> SMGKAPVDPECTAKVGKAHVYCEGNDVYDVMLNQTNLQFNNNKYYLIQLLEDDAQRNFSVWMRWGRVGKMGQHSLVACSGNLNKAKEIFQKK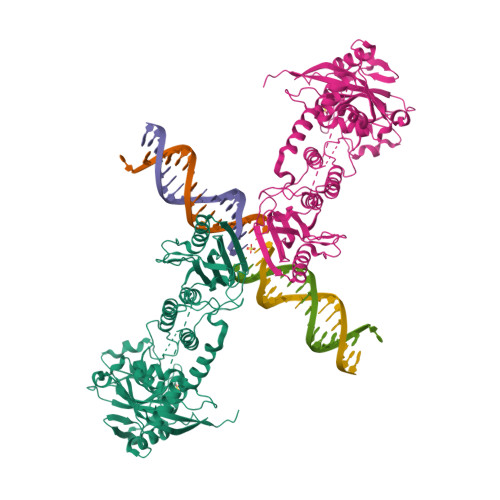FLDKTKNNWEDREKFEKVPGKYDMLQMDYATNTQDEEETKKEESLKSPLKPESQLDLRVQELIKLICNVQAMEEMMMEMKYNTKKAPLGKLTVAQIKAGYQSLKKIEDCIRAGQHGRALMEACNEFYTRIPHDFGLRTPPLIRTQKELSEKIQLLEALGDIEIAIKLVKTELQSPEHPLDQHYRNLHCALRPLDHESYEFKVISQYLQSTHAPTHSDYTMTLLDLFEVEKDGEKEAFREDLHNRMLLWHGSRMSNWVGILSHGLRIAPPEAPITGYMFGKGIYFADMSSKSANYCFASRLKNTGLLLLSEVALGQCNELLEANPKAEGLLQGKHSTKGLGKMAPSSAHFVTLNGSTVPLGPASDTGILNPDGYTLNYNEYIVYNPNQVRMRYLLKVQFNFLQLW> GAGCAGACGAG;> ACT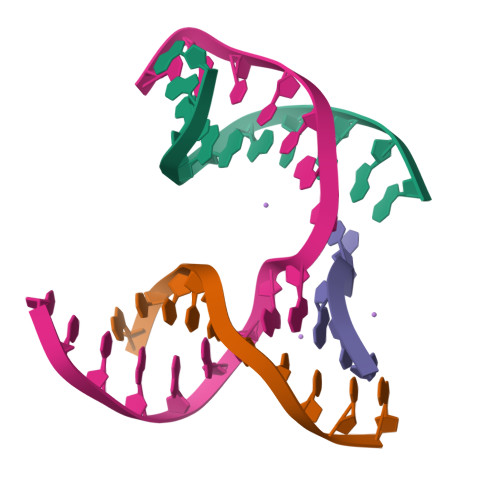CCACTCA;> CTAGT;> TCTGAGTGGCGTCTGC> EARGATEEPSPPSRALYFSGRGEQLRLRADLELPRDAFTLQVWLRAEGGQRSPAVITGLYDKCSYISRDRGWVVGIHTISDQDNKDPRYFFSLKTDRARQVTTINAHRSYLPGQWVYLAATYDGQFMKLYVNGAQVATSGEQVGGIFSPLTQKCKVLMLGGSALNHNYRGYIEHFSLWKVARTQREILSDMETHGAHTALPQLLLQENWDNVKHAWSPMKDGSSPKVEFSNAHGFLLDTSLEPPLCGQTLCDNTEVIASYNQLSSFRQPKVVRYRVVNLYEDDHKNPTVTREQVDFQHHQLAEAFKQYNISWELDVLEVSNSSLRRRLILANCDISKIGDENCDPECNHTLTGHDGGDCRHLRHPAFVKKQHNGVCDMDCNYERFNFDGGECCDPEITNVTQTCFDPDSPHRAYLDVNELKNILKLDGSTHLNIFFAKSSEEELAGVATWPWDKEALMHLGGIVLNPSFYGMPGHTHTMIHQIGHSLGLYHVFRGISEIQSCSDPCMETEPSFETGDLCNDTNPAPKHKSCGDPGPGNDTCGFHSFFNTPYNNFMSYADDDCTDSFTPNQVARMHCYLDLVYQGWQPSRKPAPVALAPQVLGHTTDSVTLEWFPPIDGHFFERELGSACHLCLEGRILVQYASNASSPMPCSPSGHWSPREAEGHPDVEQPCKSSVRTWSPNSAVNPHTVPPACPEPQGCYLELEFLYPLV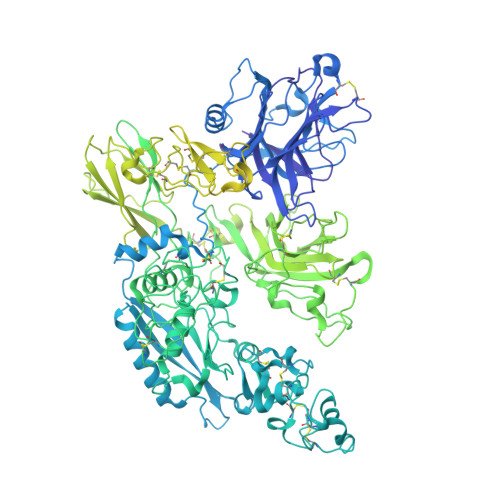PESLTIWVTFVSTDWDSSGAVNDIKLLAVSGKNISLGPQNVFCDVPLTIRLWDVGEEVYGIQIYTLDEHLEIDAAMLTSTADTPLCLQCKPLKYKVVRDPPLQMDVASILHLNRKFVDMDLNLGSVYQYWVITISGTEESEPSPAVTYIHGSGYCGDGIIQKDQGEQCDDMNKINGDGCSLFCRQEVSFNCIDEPSRCYFHDGDGVCEEFEQKTSIKDCGVYTPQGFLDQWASNASVSHQDQQCPGWVIIGQPAASQVCRTKVIDLSEGISQHAWYPCTISYPYSQLAQTTFWLRAYFSQPMVAAAVIVHLVTDGTYYGDQKQETISVQLLDTKDQSHDLGLHVLSCRNNPLIIPVVHDLSQPFYHSQAVRVSFSSPLVAISGVALRSFDNFDPVTLSSCQRGETYSPAEQSCVHFACEKTDCPELAVENASLNCSSSDRYHGAQCTVSCRTGYVLQIRRDDELIKSQTGPSVTVTCTEGKWNKQVACEPVDCSIPDHHQVYAASFSCPEGTTFGSQCSFQCRHPAQLKGNNSLLTCMEDGLWSFPEALCELMCLAPPPVPNADLQTARCRENKHKVGSFCKYKCKPGYHVPGSSRKSKKRAFKTQCTQDGSWQEGACVPVTCDPPPPKFHGLYQCTNGFQFNSECRIKCEDSDASQGLGSNVIHCRKDGTWNGSFHVCQEMQGQCSVPNELNSNLKLQCPDGYAIGSECATSCLDHNSESIILPMNVTVRDIPHWLNPTRVERVVCTAGLKWYPHPALIHCVKGCEPFMGDNYCDAINNRAFCNYDGGDCCTSTVKTKKVTPFPMSCDLQGDCACRDPQAQEHS> QASARPSSSMADFRKFFAKAKHIVIISGAGVSAESGVPTFRGAGGYWRKWQAQDLATPLAFAHNPSRVWEFYHYRRE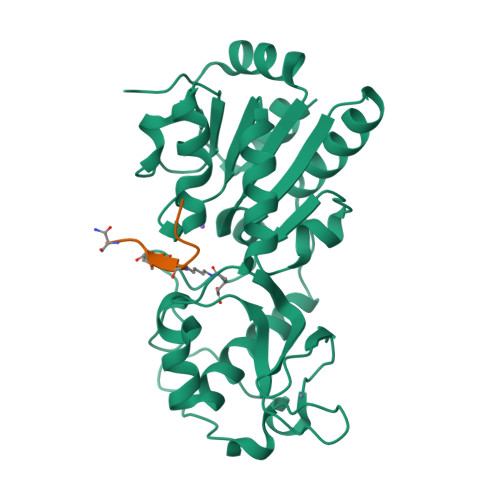VMGSKEPNAGHRAIAECETRLGKQGRRVVVITQNIDELHRKAGTKNLLEIHGSLFKTRCTSCGVVAENYKSPICPALSGKGAPEPGTQDASIPVEKLPRCEEAGCGGLLRPHVVWFGENLDPAILEEVDRELAHCDLCLVVGTSSVVYPAAMFAPQVAARGVPVAEFNTETTPATNRFRFHFQGPCGTTLPEALA;> XSAIKSYGS> VNIKTNPFKAVSFVESAIKKALDNAGYLIAEIKYDGVRGNICVDNTANSYWLSRVSKTIPALEHLNGFDVRWKRLLNDDRCFYKDGFMLDGELMVKGVDFNTGSGLLRTKWTDTKNQEFHEELFVEPIRKKDKVPFKLHTGHLHIKLYAILPLHIVESGEDCDVMTLLMQEHVKNMLPLLQEYFPEIEWQAAESYEVYDMVELQQLYEQKRAEGHEGLIVKDPMCIYKRGKKSGWWKMKPE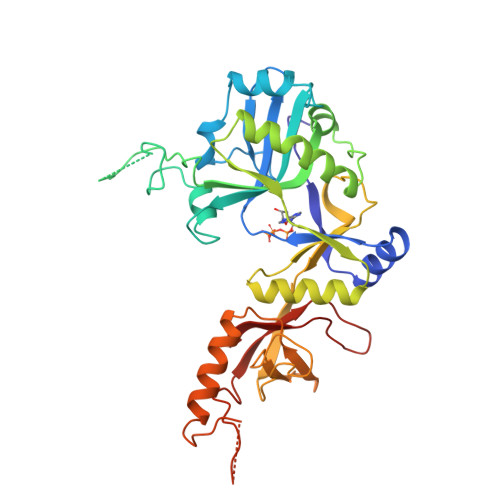NEADGIIQGLVWGTKGLANEGKVIGFEVLLESGRLVNATNISRALMDEFTETVKEATLSQWGFFSPYGIGDNDACTINPYDGWACQISYMEETPDGSLRHPSFVMFR> INLSNKTDENTISFFDSGDPERMNNEALMRGCGEQIVNLRPLLRTF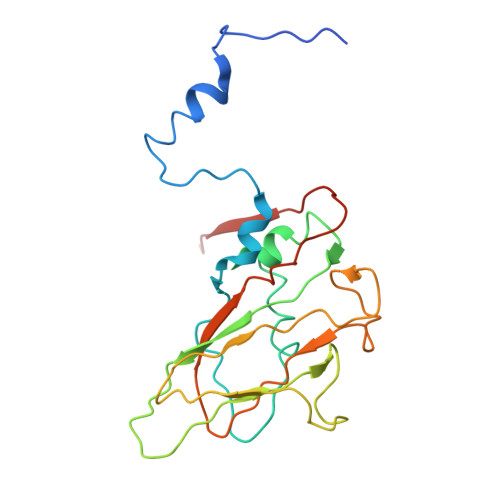RTINDNWSLAANTKTPITDLTNTADAEGRDYMSYLSFLYRFYRGGRRYKFFNTTPLKQSQTCYVRSFLIPRNYTADEINTDGPSHITYPVINPVHEVEVPFYSQYRKIPIASTSDKGYDSSLMYYTNVGTQQIVARAGNDDFTFGWMIGTPQLQGITKEVAN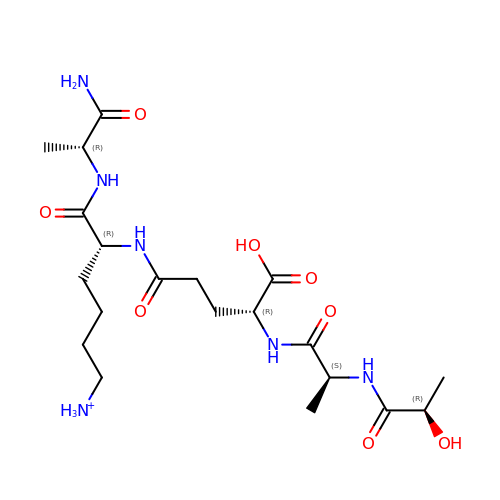[6-[[(2~{R})-1-azanyl-1-oxidanylidene-propan-2-yl]amino]-6-oxidanylidene-5-[[(4~{R})-5-oxidanyl-5-oxidanylidene-4-[[(2~{S})-2-[[(2~{R})-2-oxidanylpropanoyl]amino]propanoyl]amino]pentanoyl]amino]hexyl]azanium | C20 H37 N6 O8 | NEROIIRQSNQGCX-XVIXHAIJSA-O> GAMASGKVVKFSYMWTINNFSFCREEMGEVIKSSTFSSGAN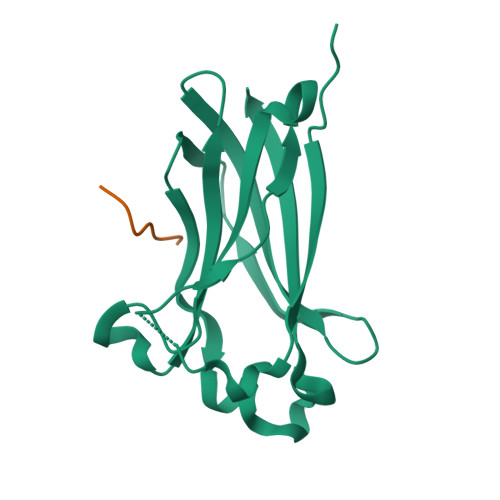DKLKWCLRVNPKGLDEESKDYLSLYLLLVSCPKSEVRAKFKFSILNAKGEETKAMESQRAYRFVQGKDWGFKKFIRRDFLLDEANGLLPDDKLTLFCEVSVVQD;> KADTTTPTT> MKTNPLPATPSVWGGSTVELPPTTRDTAGQGLLRRVLRPPISRRDGPVLPRGSGPRRAASTLWLLGLDGTDAPPGALTPNDDTEQALDKILRGTMRGGAALIGSPRHHLTRQVILTDLCQPNADRAGTLLLALRHPADLPHLAHQRAPPGRQTERLGEAWGQLMEATALGSGRAESGCTRAGLVSFNFLVAACAASYDARDAADAVRAHVTANYRGTRVGARLDRFSECLRAMVHTHVFPHEVMRFFGGLVSWVTQDELASVTAVCAGPQEAAHTGHPGRPR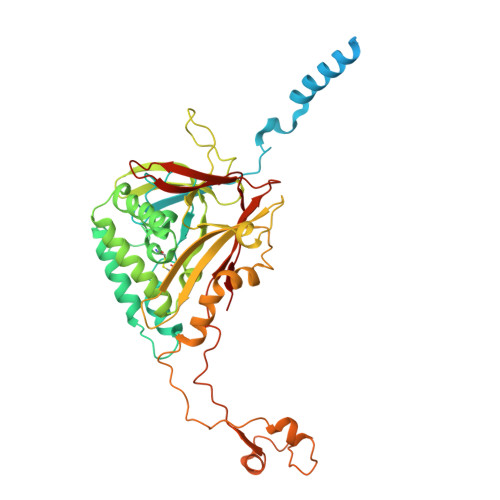SAVILPACAFVDLDAELGLGGPGAAFLYLVFTYRQRRDQELCCVYVIKSQLPPRGLEPALERLFGRLRITNTIHGTEDMTPPAPNRNPDFPLAGLAANPQTPRCSAGQVTNPQFADRLYRWQPDLRGRPTARTCTYAAFAELGMMPEDSPRCLHRTERFGAVSVPVVILEGVVWRPGEWRACA>LMLHKRNICPIKGCGKNFFSHKYLVQHQRVHSDDRPLKCPWKGCKMTFKWAWSRTEHIRVHTGARPYVCAEPDCGQTFRFVSDFSRHKRKTGHSVKKTNKR[2x]

The RELATIVE OF EARLY FLOWERING 6 protein (REF6/JMJ12), a Jumonji C (JmjC) domain—containing histone demethylase, specifically demethylates H3K27me3 at its target loci. REF6 has intrinsic DNA-binding ability and specifically recognizes its target sequence (CTCTGYTY motif, Y = T or C) via tandem zinc-finger (ZnF) domains located at its C-terminus. ZnF domains adopt the canonical ββα fold, with a small β-sheet packed against a helix in a globular structure, and wrap more than one turn of the DNA double helix, interacting with DNA in the major groove with a classic α-helix. Structural analysis demonstrates that CHG methylation is unfavorable for REF6 binding and attenuates REF6-binding affinity.

Although the overall structures of the REF6 ZnF domains were similar between complexes with methylated or unmethylated DNA oligos, there are minor conformational changes when DNA strands carrying the methyl-group. Further analysis by isothermal titration calorimetry (ITC) between REF6-ZnFs and the DNA probes with or without 5mCs revealed that 5mCs lead to great reduction in the binding affinity to the CTCTGYTY motif. In combination with EMSA assay, the biochemical and structural studies demonstrated that DNA methylation at the CTCTGYTY-motif, especially at the CTG core, is sufficient to abolish (or severely attenuate) the affinity of REF6-ZnF for this DNA sequence.>[6x]G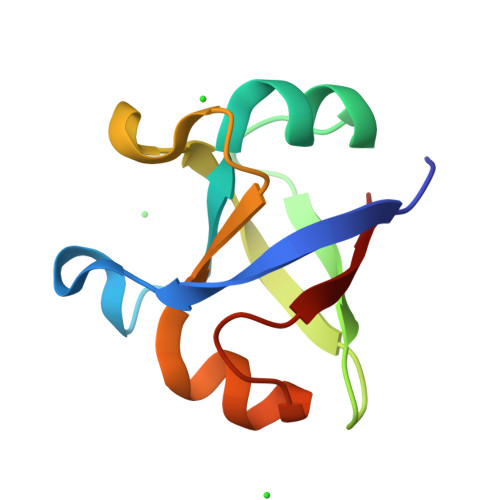PPIKLRVMEAYPEDVGKGIVRMDKASRDKLGVSAGDLVEIKGSKTPIKLRVMEAYPEDVGKGIVRMDKASRDKLGVSAGDLVEIKG> MSLKVGGLDVVGVFVGDAAATIYVGAMRIWPPVPDFTPFT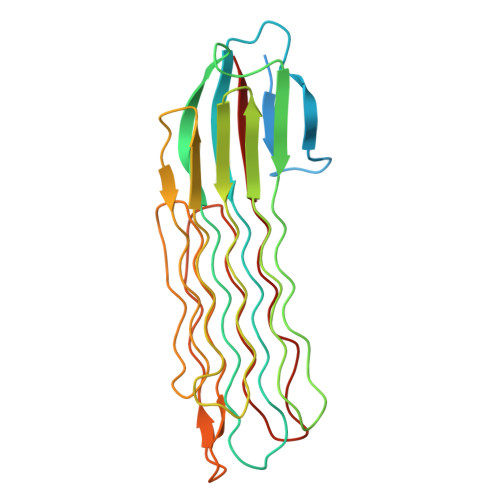ISSEDPGYEDLIDEQVPEGASGCWVTLGGAGGGGGSGRRANSGYRYGGGGGGGGGYIDRVWIPRASLGSTFTLIRGLGGAGGARAAGSSNGNNGAPGGSTVFSSGSVSLTASGGAAGVKGTSSSASGSGGAGGTTSISGVSATGYTGGKGGNGGSSPSSGQSRTDGSGAGGGGGGGVRSNDNSFSGGSNGTSSGPAGNGGRGTDGSINTGGSNAGSGGDGYVLIEWE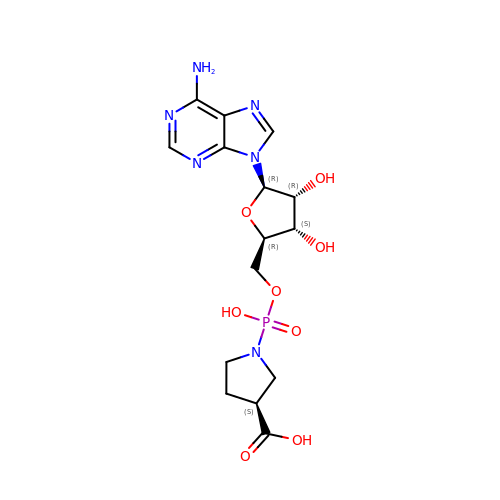5'-O-[(S)-[(3S)-3-carboxypyrrolidin-1-yl](hydroxy)phosphoryl]adenosine | C15 H21 N6 O8 P | XUGWBNVYRBVAFE-TWBCTODHSA-N>[2x]SFRDNLKVYIESPESYKNVIYYDDDVVLVRDMFPKSKMHLLLMTRDPHLTHVHPLEIMMKHRSLVEKLVSYVQGDLSGLIFDEARNCLSQQLTNEALCNYIKVGFHAGPSMNNLHLHIMT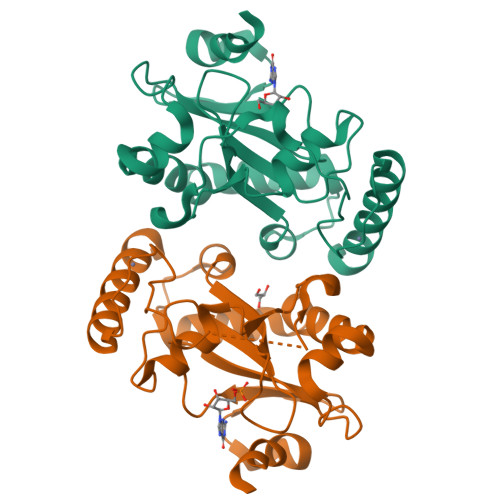LDHVSPSLKNSAHYISFTSPFFVKIDTPTSNLPTRGTLTSLFQEDLKCWRCGETFGRHFTKLKAHLQEEYDDWLDKSVSM> MSTPIPTPGRNPLQGRTPSQAHGAAGTPPVSTPFSAAQAVFSPNGPRSSPQQFKRSPATVGSTTATGGRPPSAINFDSPSASAALGALQPMTPGMDMTIRSLANLGRASEDERAKRLEEVIHILSKSKGLVSEAGLERLARSLELEFMWESSMGSDNKRTLIVAGSALEL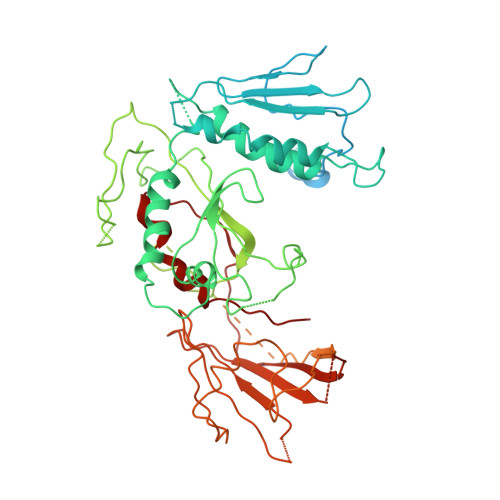LVEFSQDVVQSVTLNFPDSPEIVTKHAQKAGEILFNDLRLAPGQSPLTKSLARFAANFERLAVLDKLSILPGLNLYEAVADVYESLARLHAWELQKLREDPSLAGKDDEYLENLVLCTKSGKPAMNDRGRVGLALDYWKEKHLLRTPEAEVASWIADNERTWSILIGCAPLRDLSINPVRISDKWIGPNVVKTSLPDGLHTGEPIIDWLDPEPTFIPATDQQQQQQQQQQQQQQQQQQQQQADAPLLPPRLPEVAFHAVFDPPVHIPINLWQHLQEMGCVLPDETATQPFQQHHFRSFDSLVIPPPQGKETDATETRVFSCRKKTPFVPRRSGVRNGEGATQKMEYRIHQNTLFVPKPVMCRTLTEMSFSHPQQLVSILPYLRQYAFLAQLLENSFKPGPALQLPTDPNADTTTSKPTPNAKASHKKLDDFEAFLAKHSSHSGPISNMTPSQHQPSSDLSIDVTLRLVLPSPKLQIVFPLHATSKEEVKGKIAHVTFAVRENGRLEVEMQNMIEEEGDQMEGVKTEGDEDGEEKKRRRPQPGDLARALEVLEDVGKWAEFVRTRWV>[2x]MSLNRVFIVDDDTLTCNLLKTIVEPIFGNVEAFQHPRAFLTLSLNKQDIIILDLMMPDMDGIEVIRHLAEHKSPASLILISGYDSGVLHSAETLALSCGLNV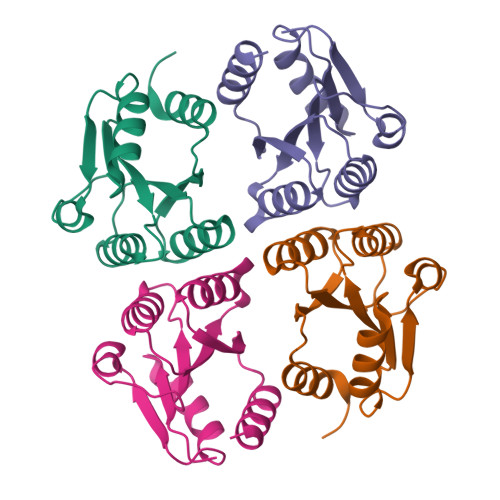INTFTKPINTEVLTCFLTSLSNRQAEGHHHHHH>[6x]MPNTIRLHRV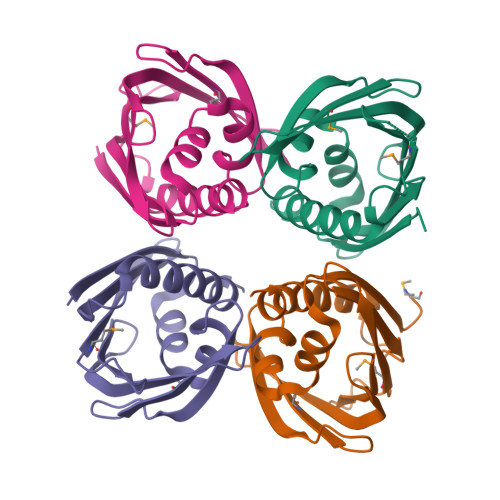LSAPPERVYRAFLDPLALAKWLPPEGFVCKVLEHDARVGGAYKMEFLAFASGQKHAFGGRYLELVPGERIRYTDRFDDAGLPGDMITTITLAPLSCGADLSIVQEGIPDAIPPENCYLGWQQSLKQLAALVEPDMPG> EQKVVAGYFADWQYANAENPYTVKDIPADKLTHVIYAFLSMCGPHTGASETVQNLVAKQCEGKDPYTAIIVDTEAALEKNFGAVSVNVPYKGHFAQLAEMKKQHPDLKILPSFGGWTMSEPFHAMA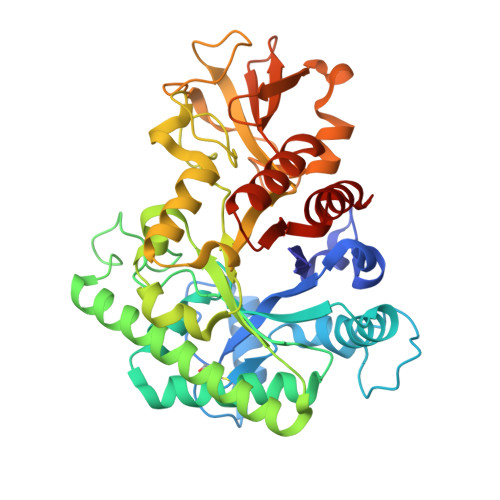KNKQAMDQFSKSAVELIAQYDFFDGIDLDWEYPGGGGLTTSPWNPDTKLSDEQKASEREAFTYLVKTMRAELDELTNQTKREYELSTAVGVGPKAAGIDWKAAEPYLTNMFAMTYDFLGGWGQQTGHTTNLHATERSWWGMGADVFINQMIELGIPSEKLVIGAAFYGRGWQGTKDFSGGLPTQDLVSEQGAQFGTGENGYFMFWDLVKNYGAKQGYEYKYDEQSQAPYLWNPEKKVFISYEDQRSIKAKANWAKQANLGGIFTWELSGDPKGELVEVMYQEMQK>[2x]MDKQYPVRQWAHGADLVVSQLEAQGVRQVFGIPGAKIDKVFDSLLDSSIRIIPVRHEANAAFMAAAVGRITGKAGVALVTSGPGCSNLITGMATANSEGDPVVALGGAVKRADKAKQVHQSMDTVAMFSPVTKYAIEVTAPD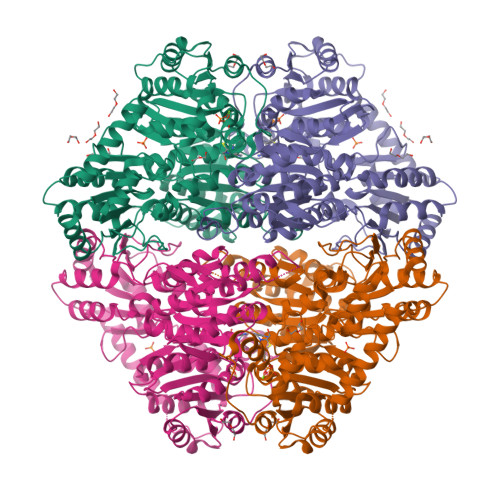ALAEVVSNAFRAAEQGRPGSAFVSLPQDVVDGPVSGKVLPASGAPQMGAAPDDAIDQVAKLIAQAKNPIFLLGLMASQPENSKALRRLLETSHIPVTSTYQAAGAVNQDNFSRFAGRVGLFNNQAGDRLLQLADLVICIGYSPVEYEPAMWNSGNATLVHIDVLPAYEERNYTPDVELVGDIAGTLNKLAQNIDHRLVLSPQAAEILRDRQHQRELLDRRGAQLNQFALHPLRIVRAMQDIVNSDVTLTVDMGSFHIWIARYLYTFRARQVMISNGQQTMGVALPWAIGAWLVNPERKVVSVSGDGGFLQSSMELETAVRLKANVLHLIWVDNGYNMVAIQEEKKYQRLSGVEFGPMDFKAYAESFGAKGFAVESAEALEPTLRAAMDVDGPAVVAIPVDYRDNPLLMGQLHLSQILEHHHHHH>GPGYQDPNSSLLEALNVRVVGSGEKVLVLAHGVGTDQSAWQRILPYFVRDHRVVLYDLVCAGSVNPDYFDFRRYTSLDAFVDDLLAILDALRLGRCTYVGHSVSASIGILASIRRPDLFAK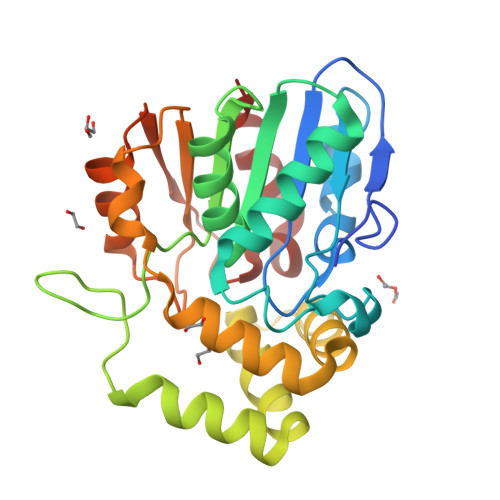LILIGASPRFLNDKNYHGGFADGEIDTVFAAMEANYAAWVSGFAPLAVGADVPEAVREFSRTLFNMRPDITLFVSRMVFNSDLRGVLGLVTVPCSVLQTSKDHSVPESMAAYLKENLGGRTTVHMLDIEGHLPHLSAPNLLAQELRRALPR[2x]> MRPAINRDNAFWFEAAKQRRLVIQRCAACKTLRHPPGPCCPHCGSFDWDTVEAAGTGQVYSYIVAHHPPHPAFEMPYVVALVELTEGTRLVTNLVGIAPDKIEIGMPV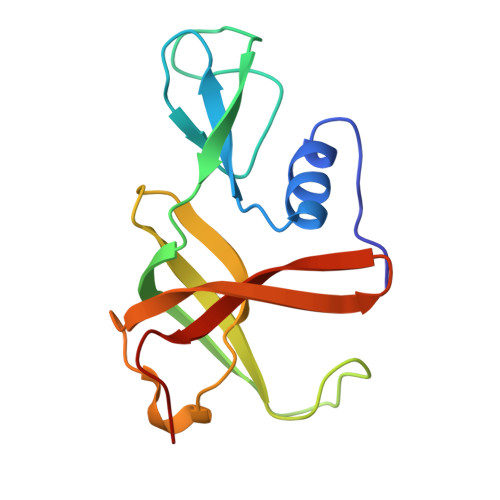VLDWLEADPELTLPVFRPAVPQEES>MSLEKEYEYLVPPDDYLAAGVHIGTQIKTGDMKKFIFKVRQDGLYVLDIRKLDERIRVAAKFLSRYEPSKILLVAARQYAHKPVQMFSKVVGSDYIVGRFIPGTLTNPMLSEYREPEVVFVNDPAIDKQAVSEATAVGIPVVALCDSNNSSADVDLVIPTNNKGRRALAIVYWLLAREIAKIRGQDFTYSIEDFEAELEGGSHHHH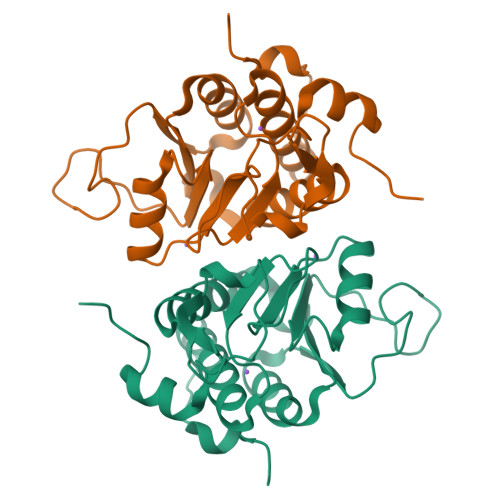HH[4x]>GPVDKTWLFGSYAWQGNPKALFLYMLVNCKETHECWWVADNEESMKSIKKSTGLKNITFTDSEKAKELFPHADVYVTENFRESYPVYMNENIKVFNTWHGVGLKHIELALGMNSVLAESIVRKYVRNYDIYKNNVLFLTTSQAMEDHFLEDMAISKELIIRGKYPRNAVYGPNGIHTYDINTLLPKNKSQYSQTILFCPTYRIGAIQGVLNSLLPDFAKLEEVCRHKNQLFIVKVHPFMKKDNYFAEMSEKYKDSEYILFWNDDYDIYEAFNSIDLAIIDYSSIFYDLLDAGVEKFIRYVPDLDEYQNDLELIGDYADLTEGRIVKSFQQLLNCLDNANIKIISTKRKQYLMDYFFGFKKENKSMESLIADVDNCQLQPKSLKELHTFDIFDTLIRRSTLRPFSIFDYVRDKAKASGIKFPLALTENWINVRNRAEHDVRDIMRKTTFERQSDKIEITLDDIYTRLQKNLLLTDEQTDFLKQAEIEAEIAHVEPIQKRINYLFSLKAKGHDVAMASDMYLPEDVIYKMLDRADTRLREIPLYLSSTIGYQKSTGKLYQHIFFDLDYQYSRWTHYGDNKHADGSVPRRLGIQTAVHDIDDFIPFENAMVNAMDNYNRYPAYQLATKMHRYRTQLVQENGFGNTLFETKYYNYAYVGASFVPYINWAIKDAIKRGYETIYFISRDGHFLKQIADKIIEIRGYNVKTKYIYGSRKAWRLPSFITKVDDETFWQFGNFVGMDSFEDLVKASYLSESELLSLFPEFESLRHAKHLRGEIAENIRKIFKNSPAYHEKVLAIAAEKRKMVRQYIQQEINPKEKFAFVEFWGRGYTQDTFGRLLNDAFGKEVKNPFYYVRSFTDDMGTSVRHNFILAPQNFSFFEPIFAQTPYDSIPDYYEEKGRIEPIINHRDRSVSDLISEGLLKFTEDYLALNTQDEDYFDAALSQFNYQYQLNTPNDQFICNVFSELKDNISSFGVEKPYAPALTLKQLESITSKQELDKLTQSIPISLSKSDVKVIDYYNKIQKNYNLPAYNSTPMRKAYAVNPLEQYVWSTQVPFRVLSLKQNSFYLDVSFAETTKRKDIFLKELNEIDVIAVDWLKGGVPRLLTEHGYITAHKDWVKKSFNDDKTNNIEEPKVKNKEKSKVLEVNTTVTNNNKQAIGKLDNNIDKSLEHHHHHH[2x]

The X-ray crystal structure of the capsule polymerase Bcs3 reveals a multi-enzyme machine adopting a basket-like shape that creates a protected environment for the synthesis of the complex Hib polymer. Supported by biochemical studies and comprehensive 2D nuclear magnetic resonance, our data explain how the ribofuranosyltransferase CriT, the phosphatase CrpP, the ribitol-phosphate transferase CroT and a polymer-binding domain function as a unique multi-enzyme assembly. The Bcs3 protomers build into a physiological and functional head-to-tail dimer, which is assembled primarily by interactions between CriT from one protomer and CroT’/CrpP’ from the neighbor protomer, with an overall basket-like shape. CroT transfers ribitol-phosphate from CDP-ribitol, generating a phosphodiester bond with the 3-OH of the nonreducing end ribose of the Hib polymer.

The crystal structure of Bcs3 (residues 1–1,115, called Bcs3-CMP hereafter) in complex with CMP was solved by molecular replacement methods using an Alphafold19 model at a maximum resolution of 2.9 Å. Bcs3-CMP crystallized in the P 212121 space group, with two molecules in the asymmetric unit and residues 1–1,115 visible in the electron density map. Region 5, the amino acids C-terminally attached to the SH3b domain, was not visible in the structure (residues 1,116–1,215). The close inspection of the electron density maps revealed a CMP molecule and glycerol located in one of the CroT protomers. The CMP binding pocket on the C-terminal side of the interdomain crevice is defined by α-helices α8, α15 and α16, loops 1–3 of the CroT-CT domain, as well as loop 4 of the CroT-NT domain. A structural comparison of the CroT protomer complexed with CMP and the apo CroT protomer reveals an important interdomain movement that has been proposed for other members of the GT-B superfamily during substrate binding and catalysis. PRTases contain a deep pocket for PRPP binding. In Bcs3-CMP, a corresponding pocket contains two phosphate groups (PO41 and PO42), is located at one end of the β-sheet, and is surrounded by α-helices α37, α38, α45 and α46, and the loops shown in Fig. 2. Structural comparison of the CriT-CAT domain with PRTases revealed that the 5-phosphate of PRPP superimposes well with PO42, whereas the β-phosphate of PRPP superimposes well with PO41. In agreement with that, a phosphate and a Zn2+ found in CrpP’s deep pocket superimpose well with substrates and Mg2+ identified in structural homologs. A structural comparison of the CroT-CMP complex with the TagFH444N-CDP-glycerol complex (PDB code 3L7K14) revealed that the CMP moieties of both structures superimpose well.> MGAVPSLTMSTTEFPTTTKRLMGWGRTAPTVASVLSTSDPEVIVRAVTRAAEEGGRGVIARGLGRSYGDNAQNGGGLVIDMPALNRIHSIDSGTRLVDVDAGVSLDQLMKAALPHGLWVPVLPGTRQVTVGGAIGCDIHGKNHHSAGSFGNHVRSMELLTANGEVRHLTPAGPDSDLFWATVGGNGLTGIILRATIEMTPTETAYFIADGDVTGSLDETIAFHSDGSEANYTYSSAWFDAISKPPKLGRAAISRGSLAKLDQLPSKLQKDPLKFDAPQLLTLPDIFPNGLANKFTFMPIGELWYRKSGTYRNKVQNLTQFYHPLDMFGEWNRAYGSAGFLQYQFVVPTEAVEEFKSIIVDIQRSGHYSFLNVFKLFGPGNQAPLSF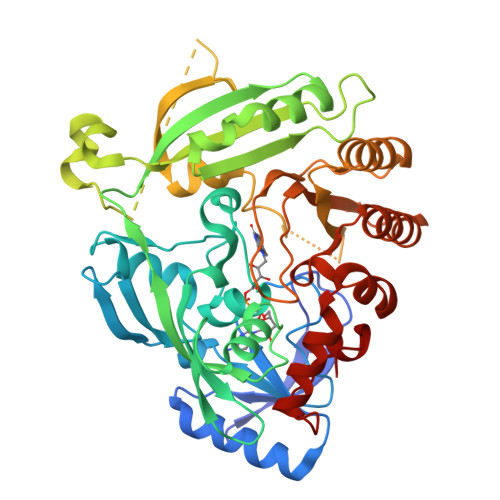PIPGWNVCVDFPIKAGLHEFVTELDRRVLEFGGRLYTAKDSRTTAETFHAMYPRIDEWIRIRRSVDPDGVFASDMARRLQLL>[2x]G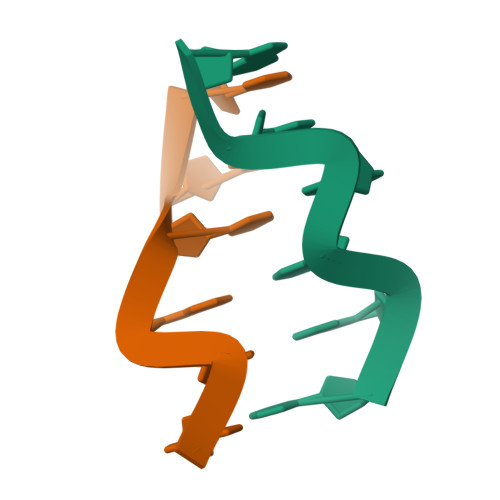CGCGCG>[6x]MSLTVKMGFIGFGKSANRYHLPYVMIRETLEVKTIFDLHVNEKAAAPFKEKGVNF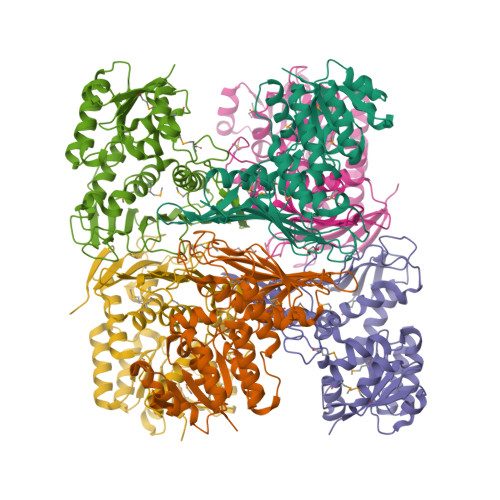TADLNELLTDPEIELITICTPAHTHYDLAKQAILAGKSVIVEKPFCDTLEHAEELFALGQEKGVVVMPYQNRRFDGDYLAMKQVVEQGFLGEINEVETHIDYYRPGSITEQGPKENGSFYGLGIHLMDRMIALFGRPDQVTYDIRNNEVSEAVDNYFDVDLHYGSKLKVKVKTNHSVASPYPRFIVHGSNGSFIKYGEDQQENDLKAGIMPDAPGFGEDSPMYYGEVTYRNGNGDWIKKQIKTPVGDYGRYYDAVYETLKNGAPQLVTKEQALTNIEILEAGFLNPSPSVYHLKENEGHHHHHH Most forms of damage to the heterocyclic nucleobases of DNA are repaired by mechanistically related pathways collectively referred to as the base-excision repair (BER) mechanism. Both the recognition of damaged sites and initiation of repair by BER are performed by DNA glycosylases, lesion-specific enzymes that recognize specific nucleobase damages in the genome and catalyze their excision through cleavage of the glycosidic bond. Among them, 8-oxoguanine (oxoG, OG) presents the greatest challenge to the DNA glycosylases responsible for its repair, due to its unique combination of structural innocuousness, extrordinary mutagenicity, and chronic low-level production. The question addressed here is whether the 8-oxoguanine DNA glycosylase responsible for oxoG recognition and repair in humans, namely hOGG1, interrogates DNA in the same way as the functionally equivalent bacterial enzyme MutM, despite the lack of an overall structural and sequence similarity between these two oxoG repair enzymes. In summary, we present X-ray crystallographic structures of human DNA glycosylase hOGG1 interrogating DNA lesions in their intrahelical position, achieved by covalent trapping of an ordinarily transient state in DNA recognition.

On the basis of this screen, we have selected the Y207C variant, because it crosslinks efficiently but is substantially distant from the active site of the enzyme to participate in the catalysis and does not interact with DNA in native LRC, and crosslinked it through the X8 linker to the minor groove N2-exocyclic amine of 3′ guanine of the target nucleobase. In parallel, we solved the structure of the control complex (2.37 Å resolution) to show that DXL between Y207C and the X8 linker does not interfere with oxoG extrusion and recognition by hOGG1. The structure of this complex, herein xLRC (with catalytically inactive K249Q), reveals that the active site as well as the overall structure is identical within an RMSD of 0.201 Å for Cα atoms (a total of 2058 atoms) to those of the native LRC16. In the xLRC structure the oxoG is extrahelical and deeply inserted into the enzyme’s lesion recognition pocket as observed in the native LRC complex, confirming that the introduced mutations and crosslinking through the X8 linker do not interfere with the extrusion of oxoG into the active site of hOGG1. Secondly, in the LRC, F319 and C253 interact with both π-faces of the extruded oxoG, which sandwich the base in the active site of hOGG1. The extruded oxoG is further stabilized by hydrogen bonding with the sidechain carbonyl of Q315 and also with the backbone carbonyl of G42. In LRC16, Y203 wedges into the DNA helical stack on the 5′-side of the estranged C stabilizing a helical bend. N149 enters the space left vacant by the oxoG extrusion and hydrogen bonds with the Watson-Crick face of the estranged C. In addition, the estranged C is stabilized by R154 and R204 that form bidentate hydrogen bonds together with N149.

> GSEGHRTLASTPALWASIPCPRSELRLDLVLPSGQSFRWREQSPAHWSGVLADQVWTLTQTEEQLHCTVYRGDKSQASRPTPDELEAVRKYFQLDVTLAQLYHHWGSVDSHFQQVAQKFQGVRLLRQDPIECLFSFICSSNNNIARITGMVERLCQAFGPRLIQLDDVTYHGFPSLQALAGPEVEAHLRKLGLGYRARCVSASARAILEEQGGLAWLQQLRESSYEEAHKALCILPGVGTQVADCICLMALDKPQAVPVDVHMWHIAQRDYSWHPTTSQAKGPSPQTNKELGNFFRSLWGPYAGWAQAVLFSADLRQ>[4x]GSCQDPTIFEERHLKYISQLGKGNFGSVELCRYDPLGDNTGALVAVKQLQHSGPDQQRDFQREIQILKALHSDFIVKYRGVSYGPGRPELRLVMEYLPS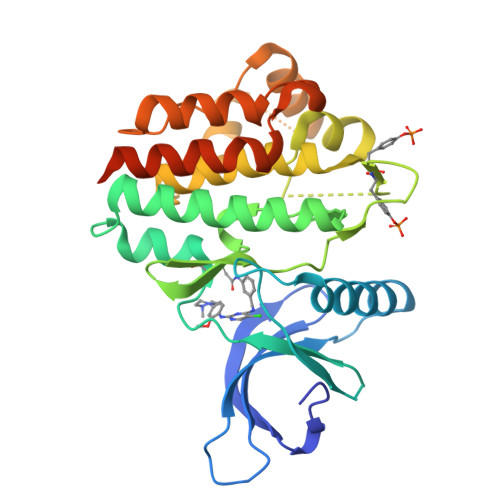GCLRDFLQRHRARLDASRLLLYSSQICKGMEYLGSRRCVHRDLAARNILVESEAHVKIADFGLAKLLPLDKDYYVVREPGQSPIFWYAPESLSDNIFSRQSDVWSFGVVLYELFTYCDKSCSPSAEFLRMMGCERDVPALCRLLELLEEGQRLPAPPACPAEVHELMKLCWAPSPQDRPSFSALGPQLDMLWSGSRGCETHAFTAHPEGKHHSLSFS>MSGQNNVVGVHYKVGRRIGEGSFGVIFEGTNLLNNQQVAIKFEPRRSDAPQLRDEYRTYKLLAGCTGIPNVYYFGQEGLHNVLVIDLLGPSLEDLLDLCGRKFSVKTVAMAAKQMLARVQSIHEKSLVYRDIKPDNFLIGRPNSKNANMIYVVDFGMVKFYRDPVTKQHIPYREKKNLSGTARYMSINTHLGREQSRRDDLEALGHVFMYFLRGSLPWQGLKAATNKQKYERIGEKKQSTPLRELCAGFPEEFYKYMH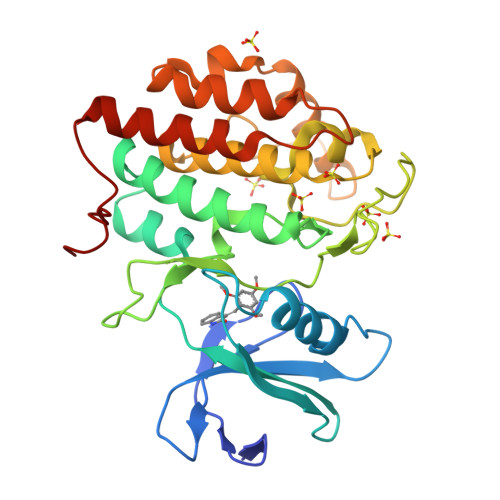YARNLAFDATPDYDYLQGLFSKVLERLNTTEDENFDWNLL[2x]> SRGPSNGQSVLENSVQ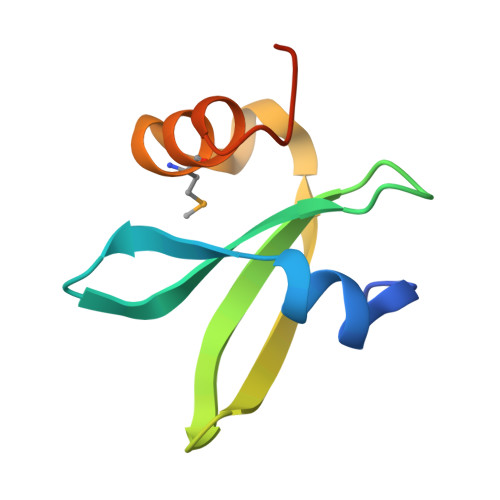VKETSPRRVSVDPQTGEFVVFDRTLGDVYHGHVRAWKDLTSDMQNALVRGGYVDRKGNPK4-{2-amino-3-[5-fluoro-2-(methylamino)quinazolin-6-yl]-4-methylbenzoyl}-1-methyl-2,5-diphenyl-1,2-dihydro-3H-pyrazol-3-one 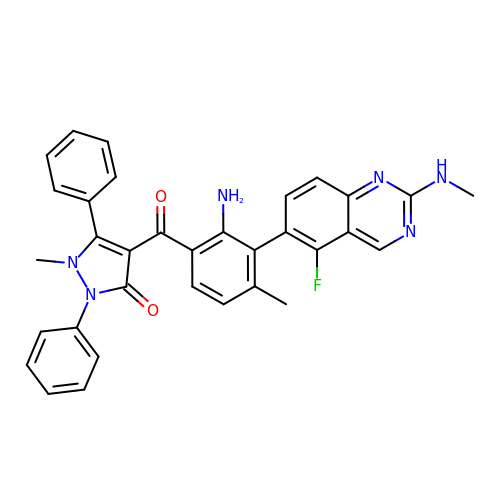| C33 H27 F N6 O2 | HBWCGZWIVPNFPT-UHFFFAOYSA-N>ILSKLATNEEHGENSPYFDGWKAYDSDPFHPLKNPNGVIQMGLAENQLCLDLIEDWIKRNPKGSICSEGIKSFKAIANFQDYHGLPEFRKAIAKFMEKTRGGRVRFDPERVVMAGGATGANETIIFCLADPGDAFLVPSPYYPAFNRDLRWRTGVQLIPIHCESSNNFKITSKAVKEAYENAQKSNIKVKGLILTNPSNPLGTTLDKDTLKSVLSFTNQHNIHLVCDEIYAATVFDTPQFVSIAEILDEQEMTYCNKDLVHIVYSLSKDMGLPGFRVGIIYSFNDDVVNCARKMSSFGLVSTQTQYFLAAMLSDEKFVDNFLRESAMRLGKRHKHFTNGLEVVGIKCL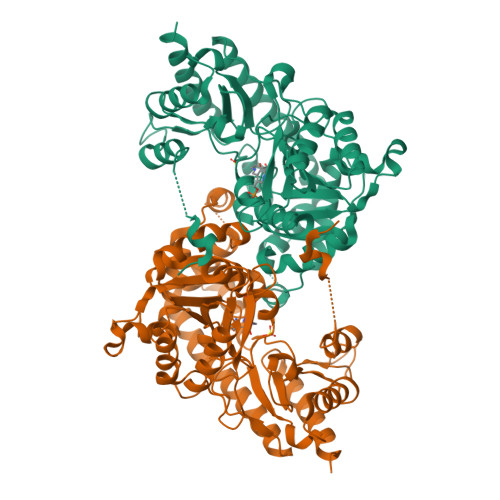KNNAGLFCWMDLRPLLRESTFDSEMSLWRVIINDVKLNVSPGSSFECQEPGWFRVCFANMDDGTVDIALARIRRFVGVEK[2x]Bacteriorhodopsin is a light-driven pump that provides proton vectorial transport across the cell membrane of the archaea. It consists of 7 transmembrane α-helices (7TM) with the retinal molecule bound covalently to the Lys 216 residue and belongs to the 7TM protein superfamily. As part of one of the simplest energy production mechanisms in the cell, bR is of great interest for bioenergetics. BR is a widely used model for expression, folding, crystallization of MPs and X-ray crystallography.

Since the expression levels of the native bR, SRII, SR1-8bRΔ(0–9), and bR0-9SRΔ(1–8) correlated with the stability of the (-4, +47) region of mRNA structure, we introduced into the wild type bR gene two silent mutations (C9A, G12A corresponding to amino acids Ala2 and Gln3) that increase the free energy by 6.2 kcal/mol and significantly reduce the stem stability. When we utilized a mild detergent for solubilization of E. coli membranes and the non-denaturing protocol for protein purification, bR expressed from the optimized gene retained its purple color. With the wild type bR, D85N and D96N mutant proteins we set up nanovolume in meso crystallization trials which yielded crystals within 5–10 days for all proteins. The crystals belonged to the spacegroup C2 with three monomers in the asymmetric unit that form a trimer. Typically for in meso crystallization, the protein molecules form membrane-like layers, with purple membrane-like packing within the layer. Despite the absence of native Halobacterium salinarum lipids, the intertrimer distance is essentially identical to that of the crystals obtained with purple membrane-derived bacteriorhodopsin. The structure of the protein and its trimer is also identical to that of purple membrane-derived bacteriorhodopsin. Data reveal the essential features of the structure, including the retinal cofactor and the hydrogen bond-linked cluster of water molecules close to the Schiff base. The growth of the first highly ordered 3D crystals of bR expressed in E. coli and the similarity of its structure to the structure of bR obtained from H. salinarum show the aptness of the presented approach for the expression of bR and its mutants suitable for all scientific and industrial applications. Our work demonstrates that bR expressed in E. coli is readily crystallized by in meso approach and, therefore, native lipids surrounding the protein are not an absolute requirement for growing well diffracting bR crystals.

>[3x]MQAQITGRPEWIWLALGTALMGLGTLYFLVKGMGVSDPDAKKFYAITTLVPAIAFTMYLSMLLGYGLTMVPFGGEQNPIYWARYADWLFTTPLLLLDLALLVDADQGTILALVGADGIMIGTGLVGALTKVYSYRFVWWAISTAAMLYILYVLFFGFTSKAESMRPEVASTFKVLRNVTVVLWSAYPVVWLIGSEGAGIVPLNIETLLFMVLDVSAKVGFGLILLRSRAIFGEAEAPEPSAGDGAAATSDGSGIEGRSGAPHHHHHHHH>MELLWCELNRDLPTPLYEQLYAHIKTEITEGRIGYGTKLPSKRKLADSLKLSQNTVEAAYEQLVAEGYVEVIPRKGFYVQAYEDLEYIRAPQAPGDALATKQDTIRYNFHPTHIDTTSFPFEQWRKYFKQTMCKENHRLLLNGDHQGEASFRREIAYYLHHSRGVNCTPEQVVVGAGVETLLQQLFLLLGESKVYGIEDPGYQLMRKLLSHYPNDYVPFQVDEEGIDVDSIVRTAVDVVYTTPSRHFPYGSVLSINRRKQLLHWAEAHENRYIIEDDYDSEFRYTGKTIPSLQSMDVHNKVIYLGAFSKSLIPSVRISYMVLPAPLAHLYKNKFSYYHSTVSRIDQQVLTAFMKQGDFEKHLNRMRKIYRRKLEKVLSLLKRYEDKLLIIGERSGLHIVLVVKNGMDE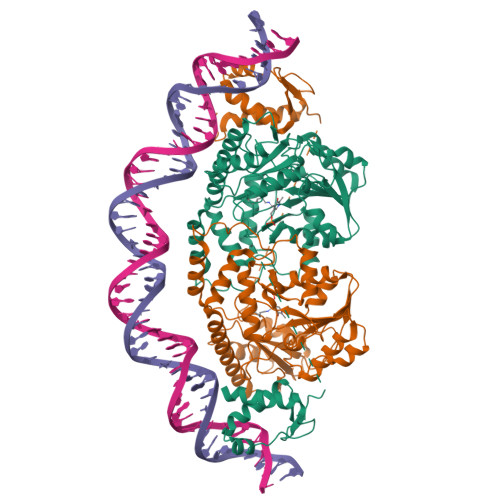QTLVEKALAAKAKVYPLSAYSLERAIHPPQIVLGFGSIPEDELEEAIATVLNAWGFLVPRGSLEHHHHHH[2x]> SKYGLQDSDEEEEEHPSKTSTKKLKTAPLPPASQTTPLQMALNGKPAPPPQSQSPEVEQLGRVVELDSDMVDITQEPVLDTMLEESMPEDQEPVSASTHIASSLGINPHVLQIMKASLLTDEEDVDMALDQRFSRLPSKADTSQEICSPRLPISASHSSKTRSLVGGLLQSKFTSGAFLSPSVSVQECRTPRAASLMNIPSTSSWSVPPPLTSVFTMPSPAPEVPLKTVGTRRQLGLVPREKSVTYGKGKLLMDMALFMGRSFRVGWGPNWTLANSGEQLNGSHELENHQIADSMEFGFLPNPVAVKPLTESPFKVHLEKLSLRQRKPDEDMKLYQTPLELKLKHSTVHVDELCPLIVPNLGVAVIHDYADWVKEASGDLPEAQIVKHWSLTWTLCEALWGHLKELDSQLNEPREYIQIL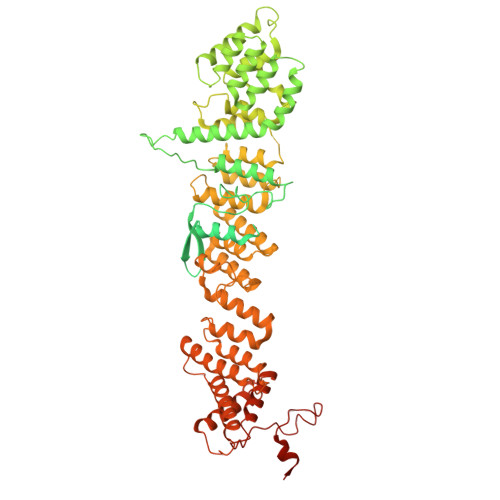ERRRAFSRWLSCTATPQIEEEVSLTQKNSPVEAVFSYLTGKRISEACSLAQQSGDHRLALLLSQFVGSQSVRELLTMQLVDWHQLQADSFIQDERLRIFALLAGKPVWQLSEKKQINVCSQLDWKRSLAIHLWYLLPPTASISRALSMYEEAFQNTSDSDRYACSPLPSYLEGSGCVIAEEQNSQTPLRDVCFHLLKLYSDRHYDLNQLLEPRSITADPLDYRLSWHLWEVLRALNYTHLSAQCEGVLQASYAGQLESEGLWEWAIFVLLHIDNSGIREKAVRELLTRHCQLLETPESWAKETFLTQKLRVPAKWIHEAKAVRAHMESDKHLEALCLFKAEHWNRCHKLIIRHLASDAIINENYDYLKGFLEDLAPPERSSLIQDWETSGLVYLDYIRVIEMLRHIQQVDCSGNDLEQLHIKVTSLCSRIEQIQCYSAKDRLAQSDMAKRVANLLRVVLSLHHPPDRTSDSTPDPQRVPLRLLAPHIGRLPMPEDYAMDELRSLTQSYLRELAVGSL> MDCSTNISPKQGLDKAKYFSGKWYVTHFLDKDPQVTDQYCSSFTPRESDGTVKEALYHYNANKKTSFYNIGEGKLESSGLQYTAKYKTVDKKKAVLKEADEKNSYTLTVL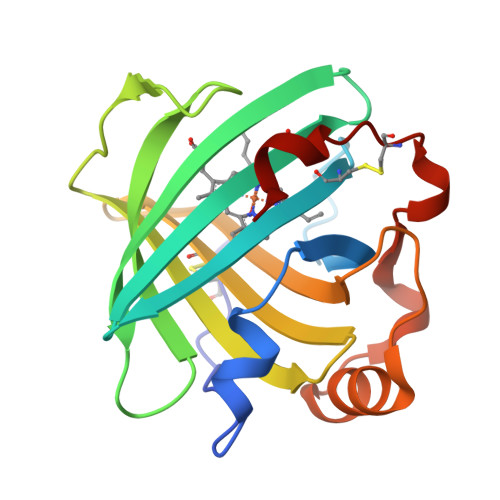EADDSSALVHICVREGSKDLGDVYTVLTHQKDAEPSAKVKSAVTQAGLQLSQFVGTKDLGCQYDDQFTSL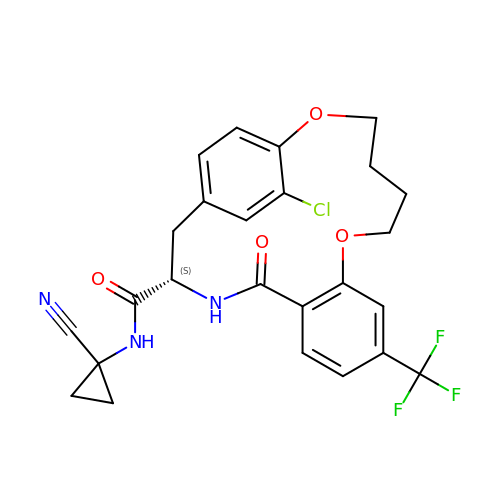(3~{S})-19-chloranyl-~{N}-(1-cyanocyclopropyl)-5-oxidanylidene-9-(trifluoromethyl)-12,17-dioxa-4-azatricyclo[16.2.2.0^{6,11}]docosa-1(21),6(11),7,9,18(22),19-hexaene-3-carboxamide | C25 H23 Cl F3 N3 O4 | XAPRSGPLBWSEHV-IBGZPJMESA-N>MQNFEIDYVEMYVENLEVAAFSWVDKYAFAVAGTSRSADHRSIALRQGQVTLVLTEPTSDRHPAAAYLQTHGDGVADIAMATSDVAAAYEAAVRAGAEAVRAPGQHSEAAVTTATIGGFGDVVHTLIQRDGTSAELPPGFTGSMDVTNHGKGDVDLLGIDHFAICLNAGDLGPTVEYYERALGFRQIFDEHIVVGAQAMNSTVVQSASGAVTLTLIEPDRNADPGQIDEFLKDHQGAGVQHIAFNSNDAVRAVKALSERGVEFLKTPGAYYDLLGERITLQTHSLDDLRATNVLADEDHGGQLFQIFTASTHPRHTIFFEVIERQGAGTFGSS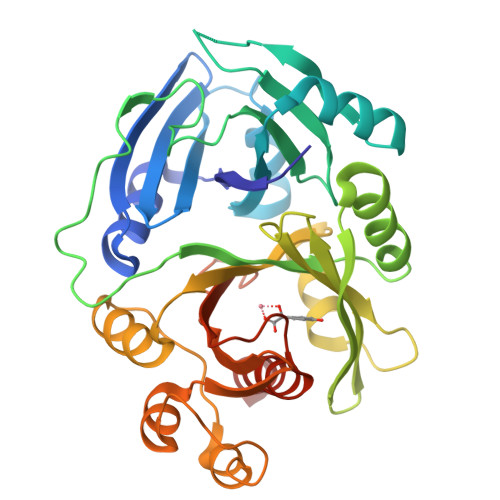NIKALYEAVELERTGQSEFGAARR[2x]> MESKRNKPGKATGKGKPVGDK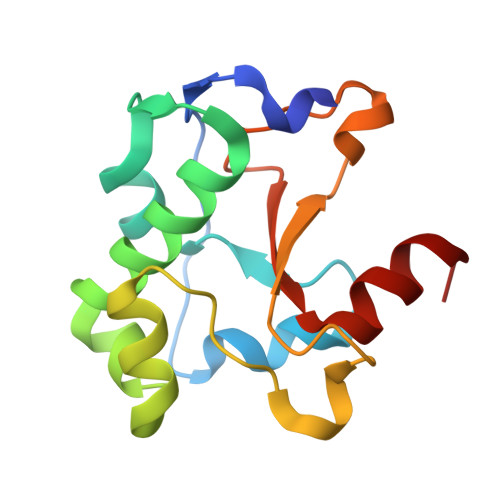WLDDAGKDSGAPIPDRIADKLRDKEFKNFDDFRKKFWEEVSKDPDLSKQFKGSNKTNIQKGKAPFARKKDQVGGRERFELHHDKPISQDGGVYDMNNIRVTTPKRHIDIHRGK>[2x]MGSSHHHHHHENLYFQGAESTQGQHNYKSLKYYYS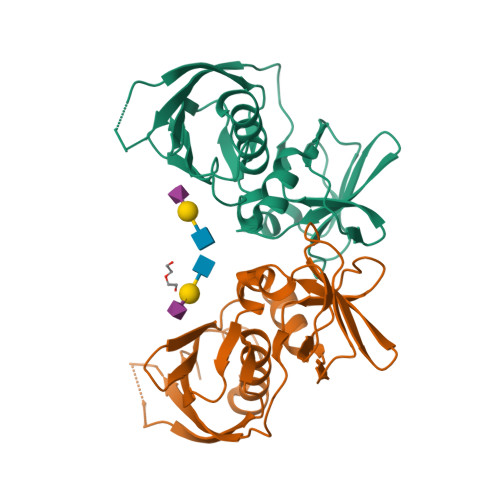KPSIELKNLDGLYRQKVTDKGVYVWKDRKDYFVGLLGKDIEKYPQGEHDKQDAFLVIEEETVNGRQYSIGGLSKTNSKEFSKEVDVKVTRKIDESSEKSKDSKFKITKEEISLKELDFKLRKKLMEEEKLYGAVNNRKGKIVVKMEDDKFYTFELTKKLQPHRMGDTIDGTKIKEINVELEYK6-(2,5-DIMETHOXY-BENZYL)-5-METHYL-PYRIDO[2,3-D]PYRIMIDINE-2,4-DIAMINE 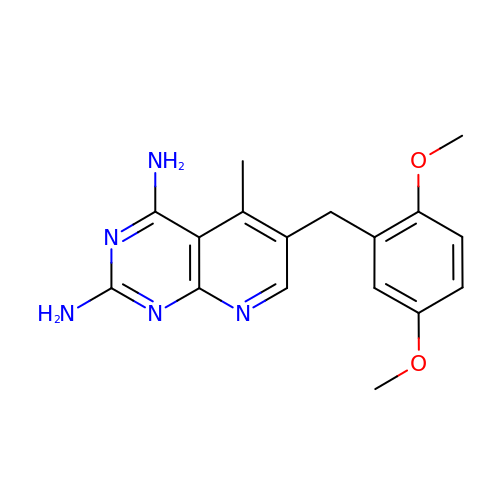| C17 H19 N5 O2 | VJXSSYDSOJBUAV-UHFFFAOYSA-N> MEEGGSTGSAGSDSSTSGSGGAQQRELERMAEVLVTGEQLRLRLHEEKVIKDRRHHLKTYPNCFVAKELIDWLIEHKEASDRETAIKLMQKLADRGIIHHVCDEHKEFKDVKLFYRFRKDDGTFPLDNEVKAFMRGQRLYEKLMSPENTLLQPREEEGVKYERTFMASEFLDWLVQEGEATTRKEAEQLCHRLMEHGIIQHVSSKHPFVDSNLLYQFRMNFRRRRRLMELLNEKSPSSQETHDSPFCLRKQSHDNRKSTSFMSVSPSKEIKIVSAVRRSSMSSCGSSGYFSSSPTLSSSPPVLCNPKSVLKRPVTSEELLTPGAPYARKTFTIVGDAVGWGFVVRGSKPCHIQAVDPSGPAAAAGMKVCQFVVS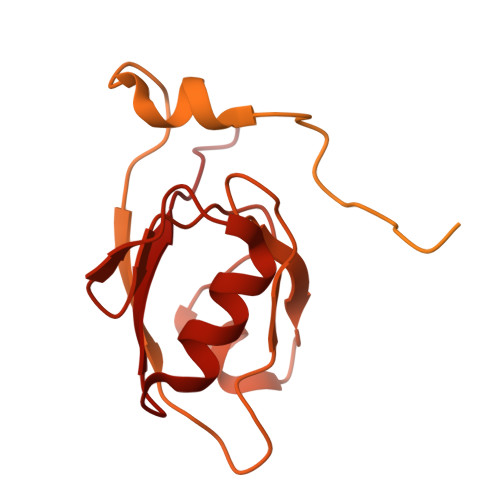VNGLNVLHVDYRTVNNLILTGPRTIVMEVMEELEC>LDGPYQ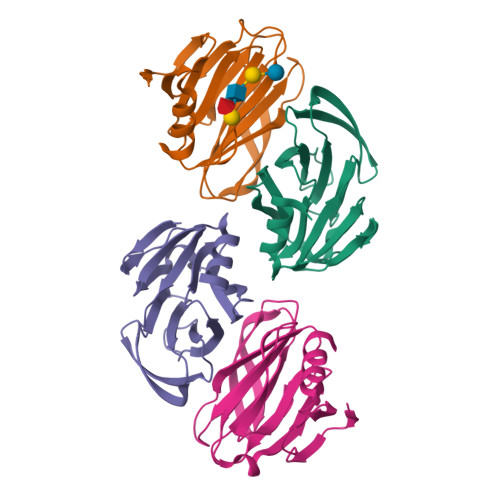PTNFKPPNDYWILLNPTNQQVVLEGTNKTDIWVALLLVEPNVTNQSRQYTLFGETKQITVENNTNKWKFFEMFRSNVSAEFQHKRTLTSDTKLAGFMKFYNSVWTFHGETPHATTDYSSTSNLSEVETVIHVEFYIIPRSQESKCSEYINTGL[4x]> MPTQKELRDTMSKKLQEAIKHPDPAVVAGRKSAIKRWVGVLQDNFMEHIKYFKGDKLKFLHNVFQDEGCWSGVRLDNAALGQRFTEEKIGGIDNPLRKYEMACSYCVVDKIHPLFQKRFESYRNKFPPGAFDGKTETEFGKYVRNSLLDSIKRKGPVFDFWIDRESGELKKYDAVEGFDSAVKFKWSEGVEYFYNHLKEEDKEKKLTEAILALSRVQSVEKDAPILDFCVNKIVDKDTLLQKLSQKDKGVYSLFVELIESCFFDTVHDLVQCWCYKEVSAGGDHSEKIFSQRDYELFLSSLSDTMLKNPELSVQARSLIMEFWECGSLYQYRKAAVNTSNYTVPTSGVFAELIVNWRREDIYKTDEEKEIEKKEILDMMSFAKDCFPEKFELFKKLIIRDLRLCGREGKRVNVDYGLFAEELFSELEKTILPPGPVGDGPCSNLRSRSKAHGSKKTTLPVDDSPQSELGTPSVSGVSSYKKKSVFTLSGNKLEHHHHHH;> MSNGDGLIRSLVDGDLEGFRQGFESFLDQCPSFLYHVSAGRFLPVFFFSMFSTAHDANILNANERVYFRFDNHGVNPRNGENRNTANLKVAVYRDGQQVVRCYSISDRPNSDGLRFSTRERNALVQEIRRQNPNLREEDLNFEQYKVCMHGKGKSQGEAIATVFEVIREKDRQGRDKFAKYSASEINLIRRLLGDHRLTIKEIEGRQLNQNQLRQLGRLVNFAQVAQGQQGIDNFMEMLASDRRQDVRDRIRREILPYITDIYNNYRQVLENNIENRNQRFEGHGFLLGFLANFSHRYTIGVDLDLSPRNSHVAFLVRHQVERENIPIVINLATRAPPYIALNRARSHAERLHVFSFIPIHTESRNTVCVGLNFNLNLDPFSVDTVGLQQDRFPLVQRLFECLENEGIRENIRDFLLHHLPAEIPRNAENYDRIFDCITGFAFGNSAFDRHPLELEEEDEAPITKYIFRHGDEGLRCLTMVFHAEGSDIVILHIRAHDAQQQGAINLQTLNVNGNDVHVWEVSCTLNNQLELDIDLPNDLGLYHDYQNNNANNFLAGDLVQVPNTENVHNTLNQVVNDGWKNIAQHRGLFQEISGALMPLVDTINVNSEDKF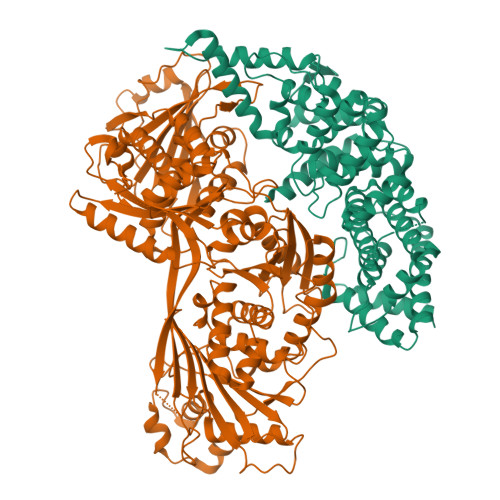RSILHGTFYASDNPYKVLAMYKVGQTYSLKRGQEEEGERVILTRITEQRLDLLLLRQPRENDLDTHPIGYVLRLANNAEEVGQQQNDARQEIGRLKKQHRGFIPITSGNEVVLFPIVFNRDAHEAGNLILFPEGIGREEHVHRLDRHVRLEHHHHHH>[4x]QFPRQCATVEALRSGMCCPDLSPVSGPGTDRCGSSSGRGRCEAVTADSRPHSPQYPHDGRDDREVWPLRFFNRTCHCNGNFSGHNCGTCRPGWRGAACDQRVLIVRRNLLDLSKEEKNHFVRALDMAKRTTHPLF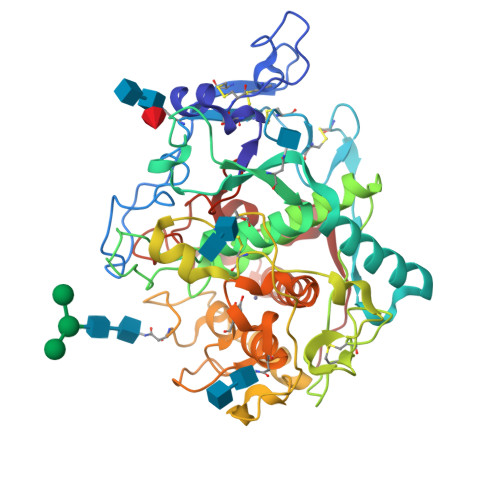VIATRRSEEILGPDGNTPQFENISIYNYFVWTHYYSVKKTFLGVGQESFGEVDFSHEGPAFLTWHRYHLLRLEKDMQEMLQEPSFSLPYWNFATGKNVCDICTDDLMGSRSNFDSTLISPNSVFSQWRVVCDSLEDYDTLGTLCNSTEDGPIRRNPAGNVARPMVQRLPEPQDVAQCLEVGLFDTPPFYSNSTNSFRNTVEGFSDPTGKYDPAVSSLHNLAHLFLNGTGGQVHLSPNDPIFVLLHTFTDAVFDEWLRRYNADISTFPLENAPIGHNRQYNMVPFWPPVTNTEMFVTAPDNLGYTYEIQWPS>[7x]MAKKTSSKGKLPPGPSPLPVLGNLLQMDRKGLLRSFLRLREKYGDVFTVYLGSRPVVVLCGTDAIREALVDQAEAFSGRGKIAVVDPIFQGYGVIFANGERWRALRRFSLATMRDFGMGKRSVEERIQEEARCLVEELRK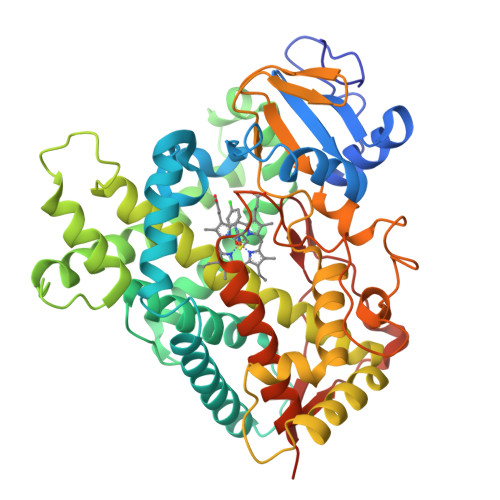SKGALLDNTLLFHSITSNIICSIVFGKRFDYKDPVFLRLLDLFFQSFSLISSFSSQVFELFSGFLKYFPGTHRQIYRNLQEINTFIGQSVEKHRATLDPSNPRDFIDVYLLRMEKDKSDPSSEFHHQNLILTVLSLFFAGTETTSTTLRYGFLLMLKYPHVTERVQKEIEQVIGSHRPPALDDRAKMPYTDAVIHEIQRLGDLIPFGVPHTVTKDTQFRGYVIPKNTEVFPVLSSALHDPRYFETPNTFNPGHFLDANGALKRNEGFMPFSLGKRICLGEGIARTELFLFFTTILQNFSIASPVPPEDIDLTPRESGVGNVPPSYQIRFLARHHHHHH> GSHMSGIALSRLAQERKAWRKDHPFGFVAVPTKNPDGTMNLMNWECAIPGKKGTPWEGGLFKLRMLFKDDYPSSPPKCKFEPPLFHPNVYPSGTVCLSILEEDKDWRPAITIKQILLGIQELLNEPNIQSPAQAEAYTIYCQNRVEYEKRVRAQAKKFAPS;> STGEPAPVLSSPPPADVSTFLAFPSPEKLLRLGPKSSVLIAQQTDTSDPEKVVSAFLKVSSVFKDEATVRMAVQDAVDALM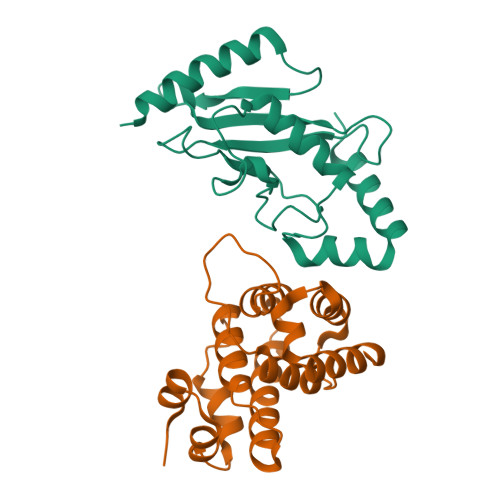QKAFNSSSFNSNTFLTRLLVHMGLLKSEDKVKAIANLYGPLMALNHMVQQDYFPKALAPLLLAFVTKPNSALESCSFARHSLLQTLYKV> MAHMVNGKVALVTGAAQGIGRAFAEALLLKGAKVALVDWNLEAGVQCKAALHEQFEPQKTLFIQCDVADQQQLRDTFRKVVDHFGRLDILVNNAGVNNEKNWEKTLQINLVSVISGTYLGLDYMSKQNGGEGGIIINMSSLAGLMPVAQQPVYCASKHGIVGFTRSAALAANLMNSGVRLNAICPGFVNTAILESIEKEENMGQYIEYKDHIKDMIKYYGILDPPL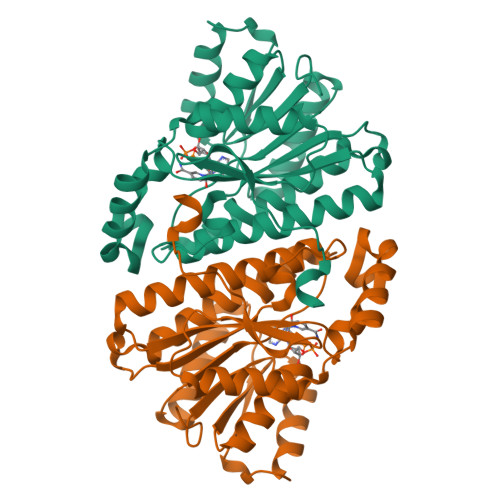IANGLITLIEDDALNGAIMKITTSKGIHFQDYGSKENLYFQ>MKKVITYGTFDLLHWGHIKLLERAKQLGDYLVVAISTDEFNLQKQKKAYHSYEHRKLILETIRYVDEVIPEKNWEQKKQDIIDHNIDVFVMGDDWEGKFDFLKDQ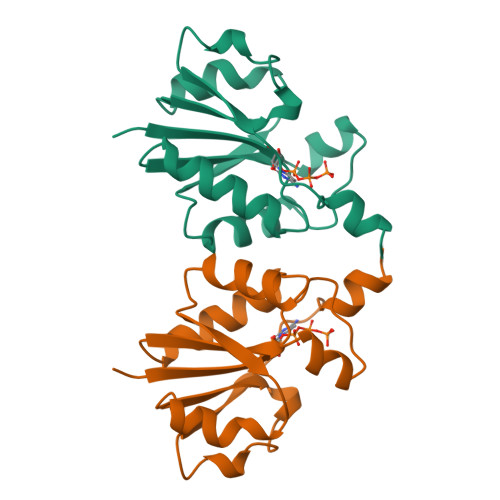CEVVYLPRTEGISTTKIKEEIAGL[2x]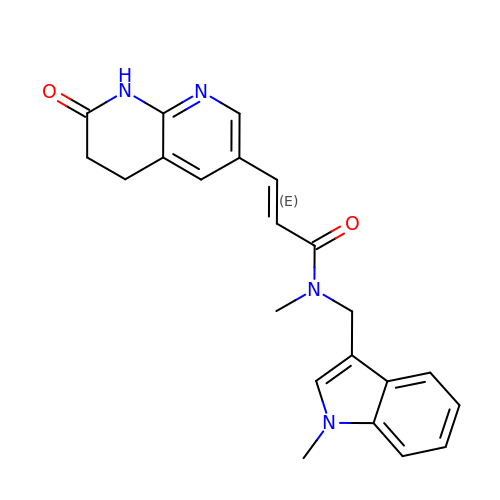(E)-N-METHYL-N-(1-METHYL-1H-INDOL-3-YLMETHYL)-3-(7-OXO-5,6,7,8-TETRAHYDRO-[1,8]NAPHTHYRIDIN-3-YL)-ACRYLAMIDE | C22 H22 N4 O2 | VAZMNDXVXVUKFY-JXMROGBWSA-N6-[3-hydroxy-2-(hydroxymethyl)prop-1-en-1-yl]-1,5-dimethylpyrimidine-2,4(1H,3H)-dione | C10 H14 N2 O4 | 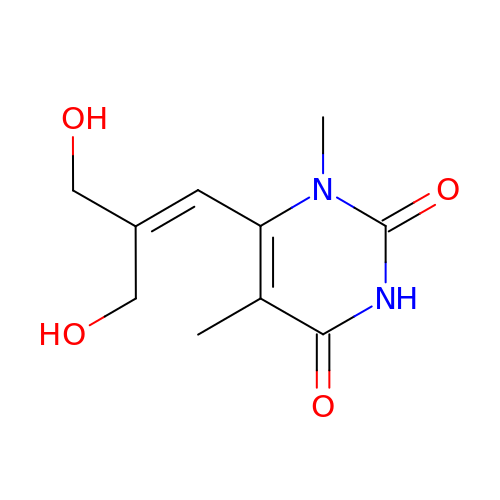BIORUVJYBNBNNA-UHFFFAOYSA-N(2S,4S)-2-[(R)-{[(2R)-2-amino-2-phenylacetyl]amino}(carboxy)methyl]-5,5-dimethyl-1,3-thiazolidine-4-carboxylic acid | C16 H21 N3 O5 S | 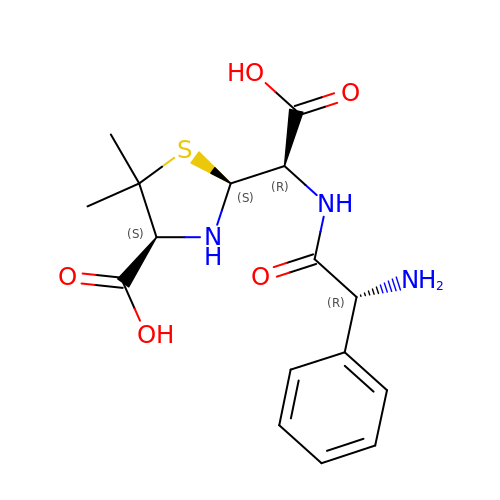KDAWOPKDXRJNHV-BLFANLJRSA-N>[3x]MRYYEKIDGSKYRNIWVVGDLHGCYTNLMNKLDTIGFDNKKDLLISVGDLVDRGAEN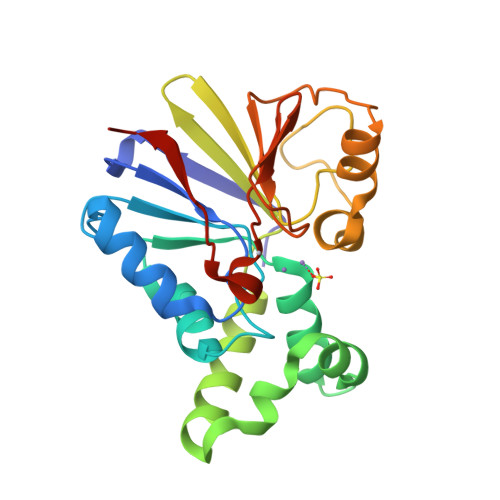VECLELITFPWFRAVRGNHEQMMIDGLSERGNVNHWLLNGGGWFFNLDYDKEILAKALAHKADELPLIIELVSKDKKYVICHADYPFDEYEFGKPVDHQQVIWNRERISNSQNGIVKEIKGADTFIFGHTPAVKPLKFANQMYIDTGAVFCGNLTLIQVQGAGA ISOEUGENOL | C10 H12 O2 | 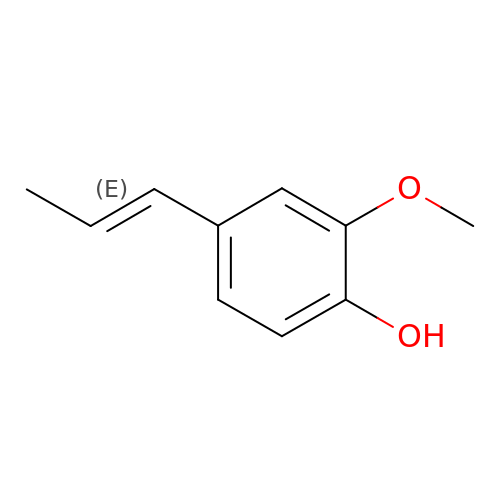BJIOGJUNALELMI-ONEGZZNKSA-N>GSNLPNQVHRKSVKKGFEFTLMVVGESGLGKSTLINSLFLTDLYPERVISGAAEKIERTVQIEASTVEIEERGVKLRLTVVDTPGYGDAINCRDCFKTIISYIDEQFERYLHDESGLNRRHIIDNRVHCCFYFISPFGHGLKPLDVAFMKAIHNKVNIVPVIAKADTLTLKERERLKKRILDEIEEHNIKIYHLPDAESDEDEDFKEQTRLLKASIPFSVVGSNQLIEAKGKKVRGR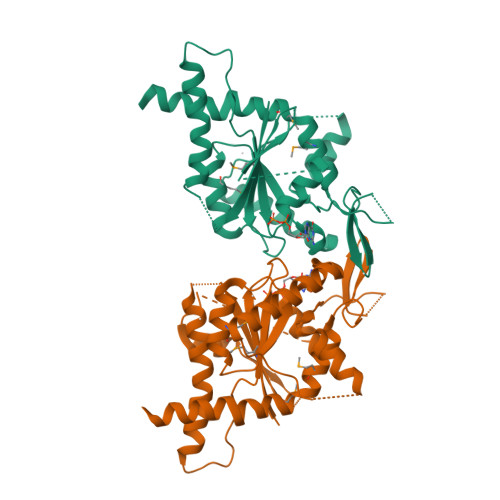LYPWGVVEVENPEHNDFLKLRTMLITHMQDLQEVTQDLHYENFRSERLKRGGRKVENEDMNKDQ[2x]Inositol-1,4,5-trisphosphate receptors (IP3Rs) are large, tetrameric cation channels that serve as the primary intracellular calcium (Ca2+) release channels in nonexcitable cells. Expressed in the endoplasmic reticulum (ER), IP3Rs mediate the flow of Ca2+ from the ER into the cytoplasm and other cellular compartments where Ca2+ contributes to the regulation of cell division, differentiation, metabolism, migration, and cell death. Notably, IP3Rs are inhibited by micromolar cytosolic Ca2+ concentrations, resulting in a biphasic dependence on Ca2+ for channel activity. Here, we collect electron cryomicroscopic images of human type 3 IP3R (hIP3R3) vitrified in a broad range of Ca2+ concentrations and treat particle abundance as a proxy for the relative free energy of each state to establish high-resolution thermodynamic models of IP3R activation and inhibition, which combined with cellular Ca2+ imaging elucidates the structural basis for IP3R-generated Ca2+ oscillations.

A fourth state shares the intact BTF ring and retracted ARM2 domain with the second and third states, but its pore is open, and its JD ring is disrupted. Based on the open conformation of the pore, we assigned the fourth state as an activated state. The Ca2+-binding profile of the activated state is the same as the preactivated+Ca2+ state, with an occupied JD site and an empty CD site. The pair-wise comparisons reveal that large changes to the ARM3-JD interface occur exclusively during the transition from the preactivated+Ca2+ to activated state: the JD-distal region of ARM3 rotates 6 Å towards the JD while the JD-proximal region shifts upwards 2 Å back to its resting state position. In the closed states, the four JDs assemble into a tetrameric ring structure. In the activated state, the contraction of the ARM3-JD interface induces a ~13˚ clockwise rigid-body rotation of the JDs that disrupts the inter-JD interactions. In the activated state, the rotation of the JD tilts S1-S4 towards the luminal side of the membrane, relaxing the belt around S6. In the activated state, rotation of the JD pulls the S6 helices away from the center of the pore, stabilizing a 13˚ bend and ~30˚ rotation about the helical axis of S6 with Gly2514 being the pivot for both. Together, the tilt and rotation of S6 reposition Phe2513 and Ile2517, which seal the pore in the closed states, out of the ion conduction pathway to create an open pore with a minimum radius of 4 Å. In addition to changing the dimensions of the pore, the tilt and rotation of S6 reorient the side chains of Arg2524, Asp2518 and Asp2522, switching the pore from an electropositive to electronegative environment that would be favorable for cation conductance.

>[4x]MSEMSSFLHIGDIVSLYAEGSVNGFISTLGLVDDRCVVEPAAGDLDNPPKKFRDCLFKVCPMNRYSAQKQYWKAKQTKQDKEKIADVVLLQKLQHAAQMEQKQNDTENKKVHGDVVKYGSVIQLLHMKSNKYLTVNKRLPALLEKNAMRVTLDATGNEGSWLFIQPFWKLRSNGDNVVVGDKVILNPVNAGQPLHASNYELSDNAGCKEVNSVNCNTSWKINLFMQFRDHLEEVLKGGDVVRLFHAEQEKFLTCDEYKGKLQVFLRTTLRQSATSATSSNALWEVEVVHHDPCRGGAGHWNGLYRFKHLATGNYLAAEENPSYKGDASDPKAAGMGAQGRTGRRNAGEKIKYCLVAVPHGNDIASLFELDPTTLQKTDSFVPRNSYVRLRHLCTNTWIQSTNVPIDIEEERPIRLMLGTCPTKEDKEAFAIVSVPVSEIRDLDFANDASSMLASAVEKLNEGFISQNDRRFVIQLLEDLVFFVSDVPNNGQNVLDIMVTKPNRERQKLMREQNILKQVFGILKAPFREKGGEGPLVRLEELSDQKNAPYQHMFRLCYRVLRHSQEDYRKNQEHIAKQFGMMQSQIGYDILAEDTITALLHNNRKLLEKHITKTEVETFVSLVRKNREPRFLDYLSDLCVSNHIAIPVTQELICKCVLDPKNSDILIRTELRPVKEMAQSHEYLSIEYSEEEVWLTWTDKNNEHHEKSVRQLAQEARAGNAHDENVLSYYRYQLKLFARMCLDRQYLAIDEISQQLGVDLIFLCMADEMLPFDLRASFCHLMLHVHVDRDPQELVTPVKFARLWTEIPTAITIKDYDSNLNASRDDKKNKFANTMEFVEDYLNNVVSEAVPFANEEKNKLTFEVVSLAHNLIYFGFYSFSELLRLTRTLLGIIDCVQGPPAMLQAYEDPGGKNVRRSIQGVGHMMSTMVLSRKQSVFSAPSLSAGASAAEPLDRSKFEENEDIVVMETKLKILEILQFILNVRLDYRISYLLSVFKKEFVEVFPMQDSGADGTAPAFDSTTANMNLDRIGEQAEAMFGVGKTSSMLEVDDEGGRMFLRVLIHLTMHDYAPLVSGALQLLFKHFSQRQEAMHTFKQVQLLISAQDVENYKVIKSELDRLRTMVEKSELWVDKKGSGKGEEVEAGAAKDKKERPTDEEGFLHPPGEKSSENYQIVKGILERLNKMCGVGEQMRKKQQRLLKNMDAHKVMLDLLQIPYDKGDAKMMEILRYTHQFLQKFCAGNPGNQALLHKHLHLFLTPGLLEAETMQHIFLNNYQLCSEISEPVLQHFVHLLATHGRHVQYLDFLHTVIKAEGKYVKKCQDMIMTELTNAGDDVVVFYNDKASLAHLLDMMKAARDGVEDHSPLMYHISLVDLLAACAEGKNVYTEIKCTSLLPLEDVVSVVTHEDCITEVKMAYVNFVNHCYVDTEVEMKEIYTSNHIWTLFENFTLDMARVCSKREKRVADPTLEKYVLSVVLDTINAFFSSPFSENSTSLQTHQTIVVQLLQSTTRLLECPWLQQQHKGSVEACIRTLAMVAKGRAILLPMDLDAHISSMLSSGASCAAAAQRNASSYKATTRAFPRVTPTANQWDYKNIIEKLQDIITALEERLKPLVQAELSVLVDVLHWPELLFLEGSEAYQRCESGGFLSKLIQHTKDLMESEEKLCIKVLRTLQQMLLKKTKYGDRGNQLRKMLLQNYLQNRKSTSRGDLPDPIGTGLDPDWSAIAATQCRLDKEGATKLVCDLITSTKNEKIFQESIGLAIHLLDGGNTEIQKSFHNLMMSDKKSERFFKVLHDRMKRAQQETKSTVAVNMNDLGSQPHEDREPVDPTTKGRVASFSIPGSSSRYSLGPSLRRGHEVSERVQSSEMGTSVLIMQPILRFLQLLCENHNRDLQNFLRCQNNKTNYNLVCETLQFLDIMCGSTTGGLGLLGLYINEDNVGLVIQTLETLTEYCQGPCHENQTCIVTHESNGIDIITALILNDISPLCKYRMDLVLQLKDNASKLLLALMESRHDSENAERILISLRPQELVDVIKKAYLQEEERENSEVSPREVGHNIYILALQLSRHNKQLQHLLKPVKRIQEEEAEGISSMLSLNNKQLSQMLKSSAPAQEEEEDPLAYYENHTSQIEIVRQDRSMEQIVFPVPGICQFLTEETKHRLFTTTEQDEQGSKVSDFFDQSSFLHNEMEWQRKLRSMPLIYWFSRRMTLWGSISFNLAVFINIIIAFFYPYMEGASTGVLDSPLISLLFWILICFSIAALFTKRYSIRPLIVALILRSIYYLGIGPTLNILGALNLTNKIVFVVSFVGNRGTFIRGYKAMVMDMEFLYHVGYILTSVLGLFAHELFYSILLFDLIYREETLFNVIKSVTRNGRSILLTALLALILVYLFSIVGFLFLKDDFILEVDRLPNNHSTASPLGMPHGAAAFVDTCSGDKMDCVSGLSVPEVLEEDRELDSTERACDTLLMCIVTVMNHGLRNGGGVGDILRKPSKDESLFPARVVYDLLFFFIVIIIVLNLIFGVIIDTFADLRSEKQKKEEILKTTCFICGLERDKFDNKTVSFEEHIKLEHNMWNYLYFIVLVRVKNKTDYTGPESYVAQMIKNKNLDWFPRMRAMSLVSNEGEGEQNEIRILQDKLNSTMKLVSHLTAQLNELKEQMTEQRKRRQRLGFVDVQNCISR> GAMGGSMGKLVQSAQNEREKLQIKIDEMDKILKKID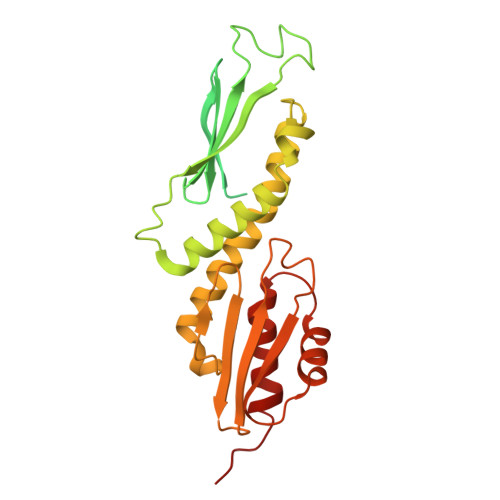NCLTEMETETKNLEDEEKNNPVEEWDSEMRAAEKELEQLKTEEEELQRNLLELEVQKEQTLAQIDFMQKQRNRTEELLDQLSLSEWDVVEWSDDQAVFTFVYDTIQLTITFEESVVGFPFLDKRYRKIVDVNFQSLLDEDQAPPSSLLVHKLIFQYVEEKESWKKTCTTQHQLPKMLEEFSLVVHHCRLLGEEIEYLKRWGPNYNLMNIDINNNELRLLFSSSAAFAKFEITLFLSAYYPSVPLPSTIQNHVGNTSQDDIATILSKVPLENNYLKNVVKQIYQDLFQDCHFYH> TAKMAFTLADRVTEEMLADKAALVVEVVEENYHDAPIVGIAVVNEHGRFFLRPETALADPQFVAWLGDETKKKSMFDSKRAAVALKWKGIELCGVSFDLLLAAYLLDPAQGVDDVAAAAKMKQYEAVRPDEAVYGKGAKRAVPDEPVLAEHLVRKAAAIWALERPFLDELRRNEQDRLLVELEQPLSSILAEMEFAGVKVDTKRLEQMGEELAEQLRTVEQRIYELAGQEFNINSPKQLGVILFEKLQLPVLKKSKTGYSTSADVLEKLAPYHEIVENILHYRQLGKLQSTYIEGLLKVVRPDTKKVHTIFNQALTQTGRLSSTEPNLQNIPIRLEEGRKIRQAFVPSESDWLIFAADYSQIELRVLAHIAEDDNLMEAFRRDLDIHTKTAMDIFQVSEDEVTPNMRRQAKAVNFGIVYGISDYGLAQNLNISRKEAAEFIERYFESFPGVKRYMENIVQEAKQKGYVTTLLHRRRYLPDITSRNFNVRSFAERMAMNTP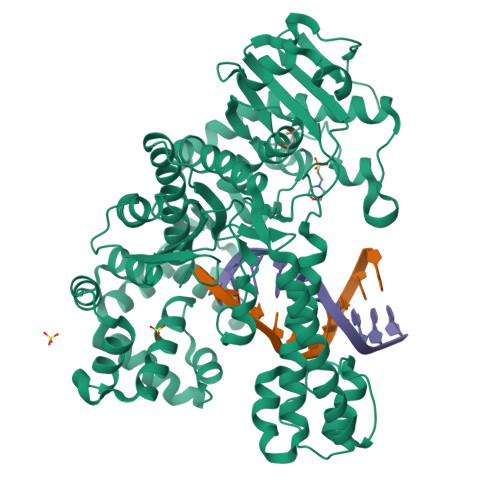IQGSAADIIKKAMIDLNARLKEERLQARLLLQVHDELILEAPKEEMERLCRLVPEVMEQAVTLRVPLKVDYHYGSTWYDAK> MSKDAFTAWNVDRRPIYSRMPKEQVGTSYHDYIATDWLTAYWDKIFIECYDKLEDLPRQFDPLQCDEEYLDFLAPLCGWTAPYW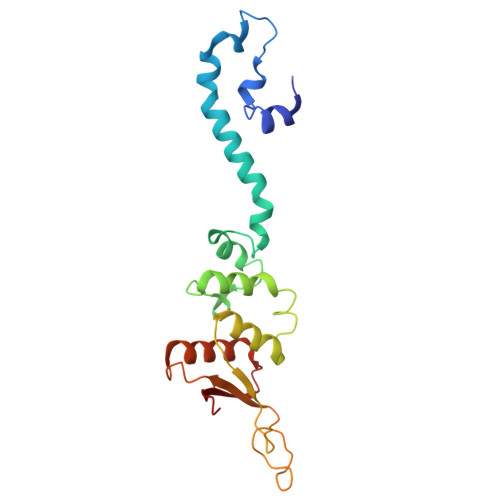SGDYPPESKRVLLANSYSLIWRDKGSLTVLSFVLNALFINHRIFVPGSFILGQSQVSEDTLGAAGWEFEILLPRDYAENGYEFRLTLKIASLFSPLWCKYRVRYDNL>MAPKCIECHINI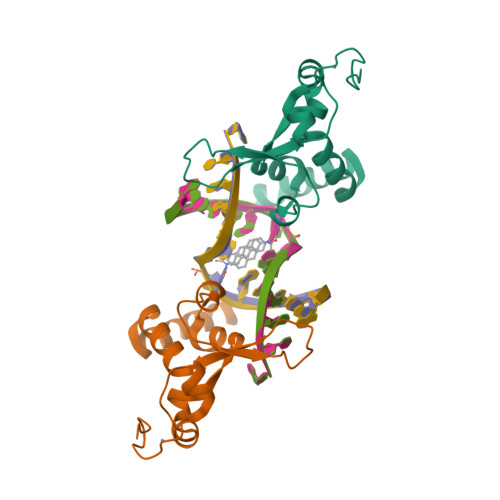EMDPVLHDVFKLQVCKQCSKEHPEKYALLTKTECKEDYFLTDPELNDEDLFHRLEKPNPHSGTFARMQLFVRCEVEAFAFKKWGGEEGLDEEWQRREEGKAHRREKKYGSAWSHPQFEK[2x]> XSNQPFNQPNVLQERQHLVNRQLVQGPNVQDAIKRVAIIFIYKNGSYRLIDYNAPEFINGYFNWRDMLYMDKPAHSNRHKEFENQIRRPDHGDSHHPELFEYPVAIMISANG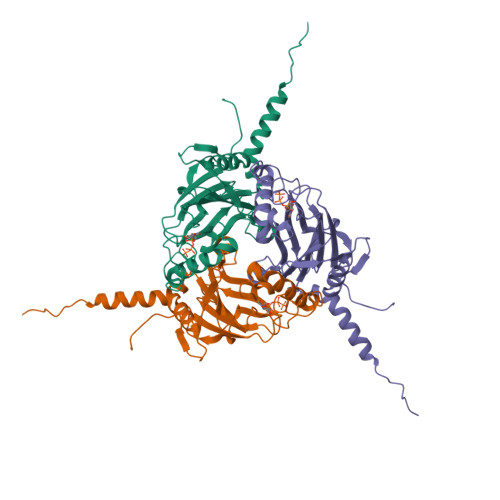NICWENVRVEVENEDCLNHEDWRRARAWGPRCYKGSQMMKCSALGRFLYIPLRCQNESLKFKFPSRMSGGDNRYSSHSIGQVIQNNIIIRNNPLYLDNEGDLIDYMQAKNLCYIDSAAVVDCNGLAGDSEC>[2x]G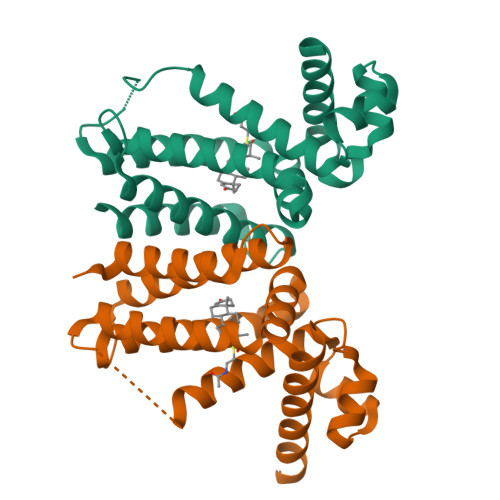AMEVAVLAESELGSEAQRERRKRILDATMAIASKGGYEAVQMRAVADRADVAVGTLYRYFPSKVHLLVSALGREFSRIDAKTDRSAVAGATPFQRLNFMVGKLNRAMQRNPLLTEAMTRAYVFADASAASEVDQVEKLIDSMFARAMANGEPTEDQYHIARVISDVWLSNLLAWLTRRASATDVSKRLDLAVRLLIGDQDSA> WSHPQFEKGAENLYFQSMTPALLGNLGVSLALAFSLLGLGLALLAYLQGDGRFLRGARALVFPAFLAALAAFLALEWALLVHDFSLAYVARNHSTKDPLWVTLVTPWAALEGSILLWGLLQTLYTLLASRKPLDPWRASLVLAVLFGIQVFFFGVMATIASPFETLPDPPPDGVGPNPLLQNHWMMAVHPVLMYLGFVGLSVPYAYAVAAMATRRYQTWVEETRWWTLIAWGFLTAGKVAGMWWSYEVLGWGGYWAWDPVENASFIPWLLATAFLHTAFVQQTRGAFKTWNFAFVTLAFAATLLGTFLTRSGIIQSVHAFAEGPVGPA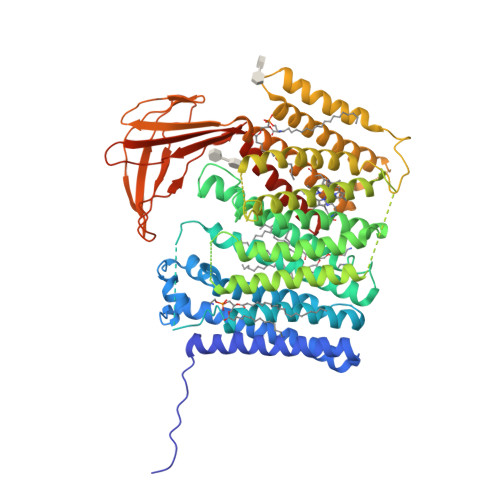FLGFFLFATGLGLGLLSRVSREVRDAALFHPLSREGALLLGAFFFAGWALVVVLGTFYPLLVEAFTGAKVSVGAPFFNQVSAPLGAGILLLMGVGPLLPWRRARGEVLRNLLVLLLALALGTLFGLLRGYTLGASFALGLFLYNAAAIYLLAREGVLARVRAGLSPWGFLANRRRVGSLVVHFAVALMGLAIAFSQTYRLESEKTLYRGEAWEVGGVRMTFQGVRALDEGRRFAVEALLKTDRFGEVRPRLHFYPQMNSPLPAPKVIYTPGNDYYFLLMDFDREKGEWASLRLIVTPLVFWMWVAGGLMALGTLYILWPAARPEEARGVSPA> PP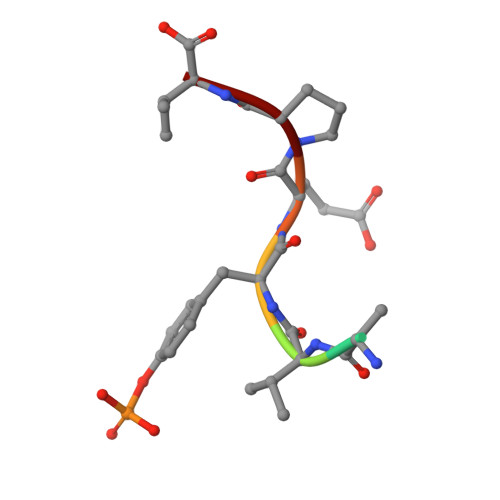VYEPV>[2x]PMILGYWNVRGLAHPIRLLLEYTDSSYEEKRYAMGDAPDYDRSQWLNEKFKLGLDFPNLPYLIDGSRKITQSNAIMRYLARKHHLCGETEEERIRADIVENQVMDNRMQLIMLCYNPDFEK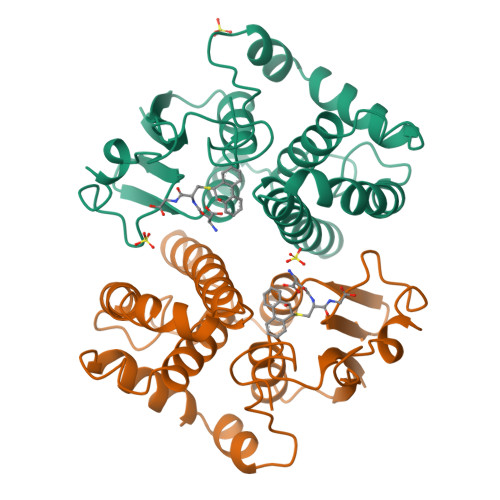QKPEFLKTIPEKMKLYSEFLGKRPWFAGDKVTYVDFLAYDILDQYHIFEPKCLDAFPNLKDFLARFEGLKKISAYMKSSRYLSTPIFSKLAQWSNK> MLAVGIVGLPNVGKSTLFNALTRAN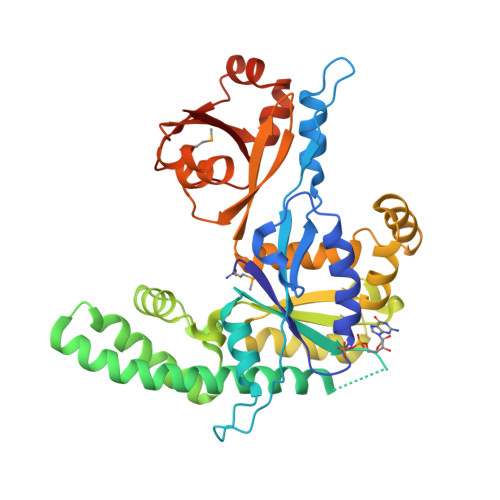ALAANYPFATIDKNVGVVPLEDERLYALQRTFAKGERVPPVVPTHVEFVDIAGLVKGAHKGEGLGNQFLAHIREVAAIAHVLRCFPDPDVVHVMGRVDPLEDAEVVETELLLADLATLERRLERLRKEARADRERLPLLEAAEGLYVHLQEGKPARTFPPSEAVARFLKETPLLTAKPVIYVANVAEEDLPDGRGNPQVEAVRRKALEEGAEVVVVSARLEAELAELSGEEARELLAAYGLQESGLQRLARAGYRALDLLTFFTAGEKEVRAWTVRRGTKAPRAAGEIHSDMERGFIRAEVIPWDKLVEAGGWARAKERGWVRLEGKDYEVQDGDVIYVLFNA> MDEIITRWATDLAKYQKEFKEQAAKVMEWDRLLVENGEKIQKLYTST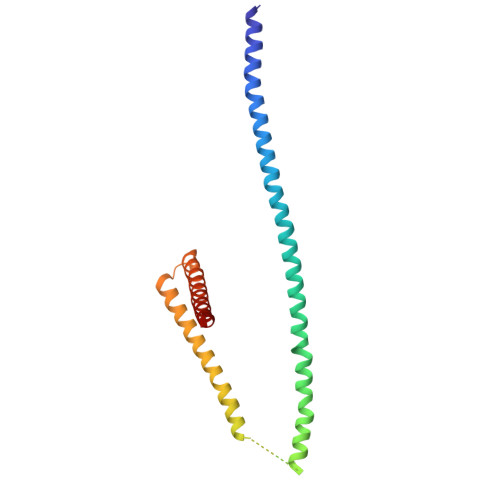YEAERASNEIERQLSNVESQQEELTAWLDRYERELDELYAKQMGSAAGEQAAGPDQERERTYKLAEKLTDQLDEMGKDLAKMIKEINDMSNTLSKGSKPDDPLTQIVRVLNGHLAQLQWIDTNAAALQAKVAAAQK>[2x]GSHMATVQQLEGRWRLVD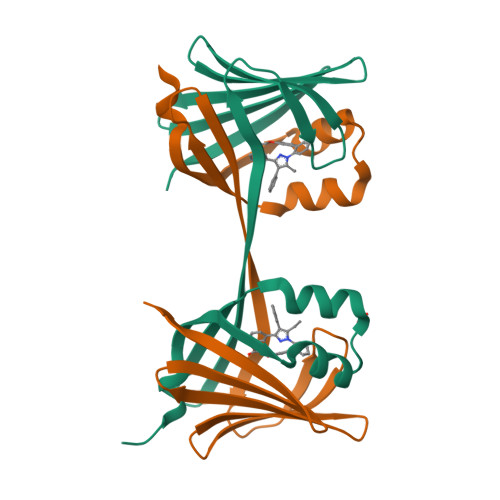SKGFDEYMKELGVGIALRKMGAMAKPDCIITCDGKNLTIKTESTLKTTQFSCTLGEKFEETTADGRKTQTVCNFTDGALVQHQEWDGKESTITRKLKDGKLVVECVMNNVTCTRIYEKVE>AYTTFSQTKNDQLKEPMFFGQPVNVARYDQQKYDIFEKLIEKQLSFFWRPEEVDVSRDRIDYQALPEHEKHIFISNLKYQTLLDSIQGRSPNVALLPLISIPELETWVETWAFSETIHSRSFTHIIRNIVNDPSVVFDDIVTNEQIQKRAEGISSYYDELIEMTSYWHLLGEGTHTVNGKTVTVSLRELKKKLYLCLMSVNALEAIRFYVSFACSFAFAERELMEGNAKIIRLIARDAALHLTGTQHMLNLLRSGADDPEMAEIAEECKQECYDLFVQAAQQEKDWADYLFRDGSMIGLNKDILCQYVEYITNIRMQAVGLDLPFQTRSNPIPWINTWLVS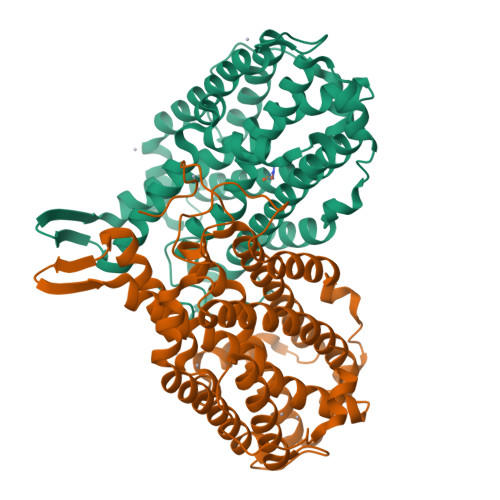DNVQVAPQEVEVSSYLVGQIDSEVDTDDLSNFQL[2x]>ARKCSLTGKWTNNLGSIMTIRAVNSRGEFTGTYLTAVADNPGNITLSPLLGIQHKRASQPTFGFTVHWNFS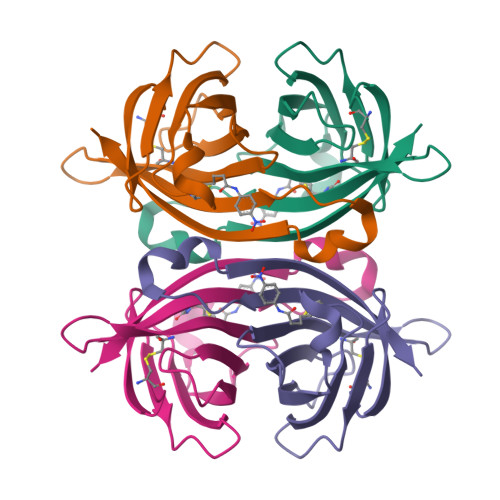ESTTVFTGQCFIDRNGKEVLKTMWLLRSSVNDISYDWIATRVGYNNFTRLSTVEE[2x]> GSHMDDDLVDAEGNLVENGGTYYLLPHIWAHGGGIETAKTGNEPCPLTVVRSPNEVSKGEPIRISSQFRSLFIPRGSLVALGFANPPSCAASPWWTVVDSPQGPAVKLSQQKLPEKDILVFKFEKVSHSNIHVYKLLYCQHDEED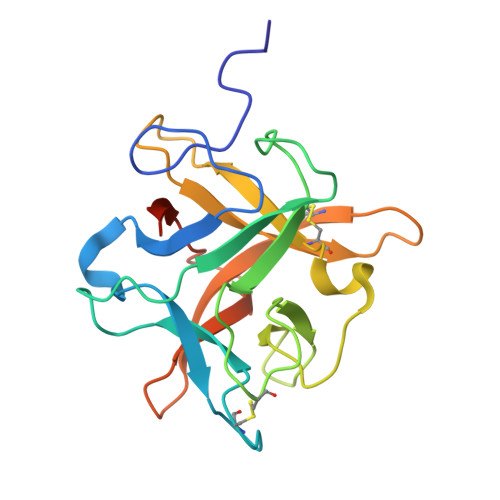VKCDQYIGIHRDRNGNRRLVVTEENPLELVLLKAKSETASSH> LTAKKRPSVVYLHNAECTGCSESVLRTVDPYVDELILDVISMDYHETLMAGAGHAVEEALHEAIKGDFVCVIEGGIPMGDGGYWGKVGGRNMYD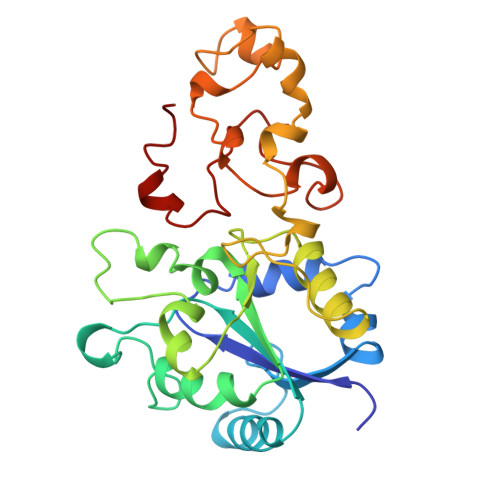ICAEVAPKAKAVIAIGTCATYGGVQAAKPNPTGTVGVNEALGKLGVKAINIAGCPPNPMNFVGTVVHLLTKGMPELDKQGRPVMFFGETVHDNCPRLKHFEAGEFATSFGSPEAKKGYCLYELGCKGPDTYNNCPKQLFNQVNWPVQAGHPCIACSEPNFWDLYSPFYSA> AGVVGAAEGFAHGVTGGGSASPVYPTTTDELVSYLGDNEPRVIILDQTFDFTGTEGTETTTGCAPWGTASQCQVAINLHSWCDNYQASAPKVSVTYDKAGILPITVNSNKSIVGQGTKGVIKGKGLRVVSGAKNVIIQNIAVTDINPKYVWGGDAITVDDSDLVWI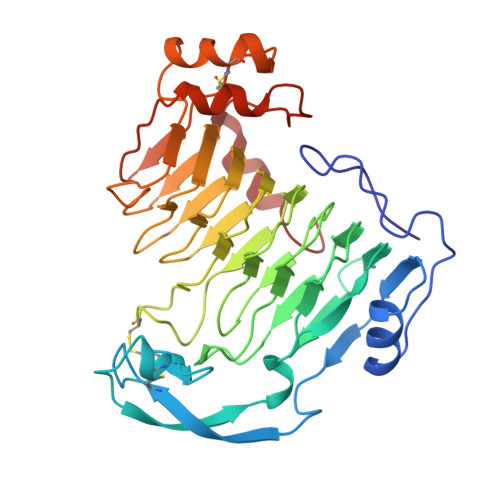DHVTTARIGRQHIVLGTSADNRVTISYSLIDGRSDYSATCNGHHYWGVYLDGSNDMVTLKGNYFYNLSGRMPKVQGNTLLHAVNNLFHNFDGHAFEIGTGGYVLAEGNVFQDVNVVVETPISGQLFSSPDANTNQQCASVFGRSCQLNAFGNSGSMSGSDTSIISKFAGKTIAAAHPPGAIAQWTMKNAGQGK PHOSPHOCHOLINE 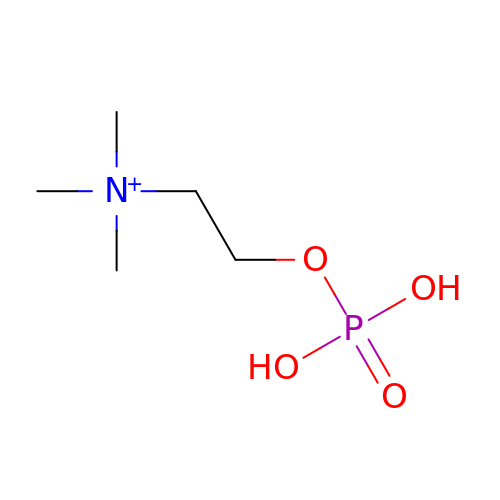| C5 H15 N O4 P | YHHSONZFOIEMCP-UHFFFAOYSA-O> MEQKNVRNFCIIAHVDHGKSTLADRLLEYTGAISEREKREQLLDTLDVERERGITVKMQAVRMFYKAKDGNTYKLHLIDTPGHVDFSYEVSRALAACEGALLLIDASQGIEAQTVANFWKAVEQDLVIIPVINKIDLPSADVDRVKKQIEEVLGLDPEEAILASAKEGIGIEEILEAIVNRIPPPKGDPQKPLKALIFDSYYDPYRGAVAFVRIFDGEVKPGDKIMLMSTGKEYEVTEVGAQTPKMTKFDKLSAGDVGYIAASIKDVRDIRIGDTITHAKNPTKEPVPGFQPAKPMVYAGIYPAEDTTYEELRDALEKYAINDAAIVYEPESSPALGMGFRVGFLGLLHMEIVQERLEREYGVKIITTAPNVIYRVKKKFTDEVIEVRNPMDFPDNAGLIEYVEEPFVLVTIITPKEYVGPIIQLCQEKRGIQKNMTYLDPNTVYLEYEMPLSEIIVDFHDKIKSISRGFASYDYEFIGYRPSDLIKLTVLINKKPVDALSFIVHADRAQKFARRVAEKLRETIPRQLFEVHIQVAKGGKVIASERIKPLRANVTAKC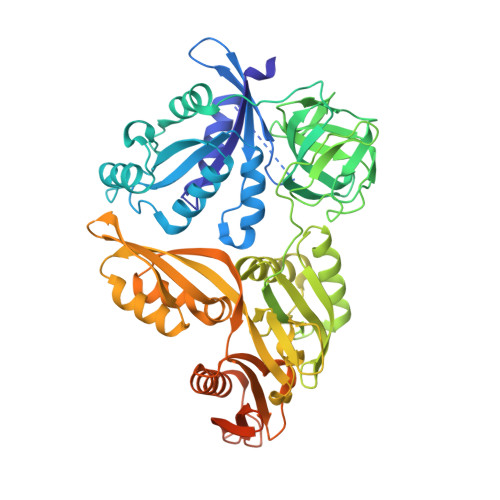YGGDVTRKKKLLENQKEGKKRMKQFGKVQLPQEAFLSVLKVE>MAFQLEMVTRETVVIRLFGELDHHAVEQIRAKISTAIFQGAVTTIIWNFERLSFMDSSGVGLV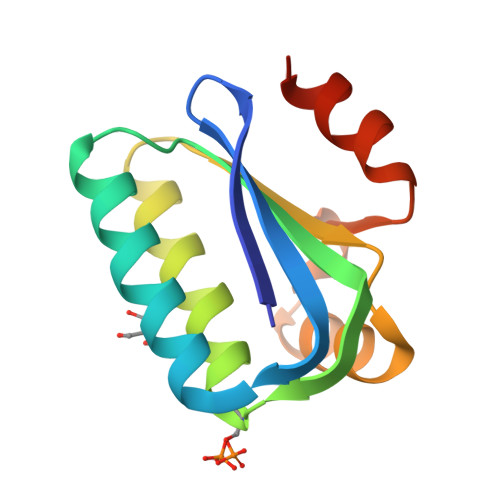LGRMRELEAVAGRTILLNPSPTMRKVFQFSGLGPWMMDATEEEAIDRVRGIVNG[2x]2-OXO-4-METHYLPENTANOIC ACID | C6 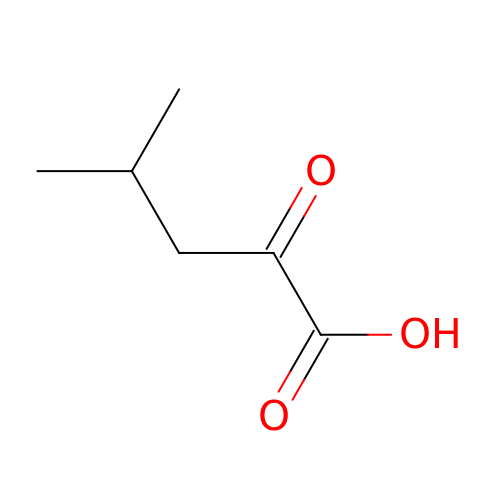H10 O3 | BKAJNAXTPSGJCU-UHFFFAOYSA-N>AGWQSYVDNLMCDGCC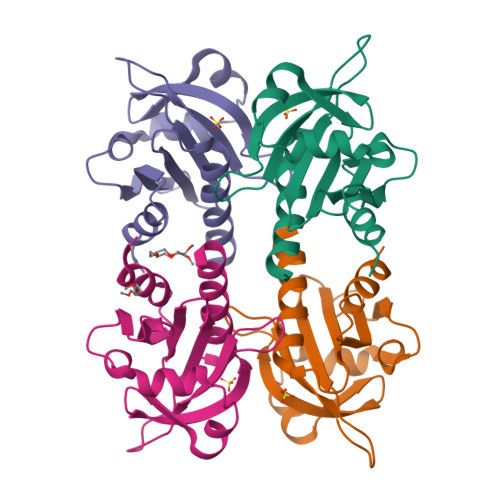QEAAIVGYCDAKYVWAATAGGVFQSITPIEIDMIVGKDREGFFTNGLTLGAKKCSVIRDSLYVDGDCTMDIRTKSQGGEPTYNVAVGRAGRALVIVMGKEGVHGGTLNKKAYELALYLRRSDV[4x]> MSADHDHDHDHDHDHKPAPMVEEVSDFEILEMAVRELAIEKGLFSAEDHRVWKDYVHTLGPLPAARLVAKAWLDPEYKKLCIEDGVEASKAVGVNWVTSPPTQFGTPSDYCNLRVLADSPTLKHVVVCTLCSCYPRPILGQSPEWYR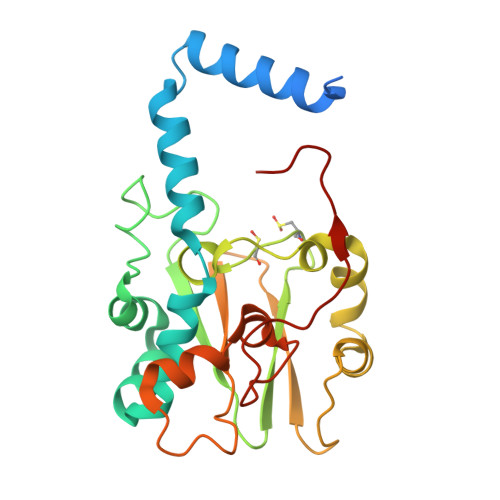SPNYRRRLVRWPRQVLAEFGLQLPSEVQIRVADSNQKTRYIVMPVRPEGTDGWTEDQLAEIVTRDCLIGVAVPKPGITVNAKRPVLKANRPVHHDH> SKQHCVKLNDGHLIPALGFGTYKPKEVPKSKSLEAACLALDVGYRHVDTAYAYQVEEEIGQAIQSAIAAGVVKREDLFITTKLWCTCFRPELVKPALEKSLKKLQLDYVDLYIMHYPVPMKSGDNDFPVNEQGKSLLDTVDFCDTWERLEECKDAGLVKSIGVSNFNHRQLERILNKPGLNYKPVCNQVECHLYLNQRKLLDYCESKDIVLVAYGALGTQRYKEWVDQNSPVLLNDPVLCDVAKKNKRSPA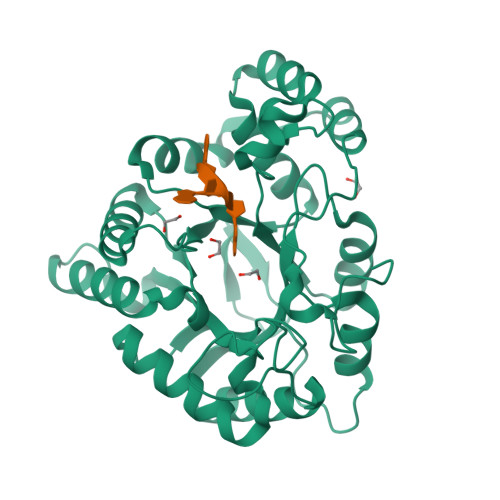LIALRYLIQRGIVPLAQSFKENEMRENLQVFGFQLSPEDMKTLDGLNKNFRYLPAEFLVDHPEYPFVEEY> QPIFLNVLEAIEPGVVCAGHDNNQPDSFAALLSSLNELGERQLVHVVKWAKALPGFRNLHVDDQMAVIQYSWMGLMVFAMGWRSFTNVNSAMLYFAPDLVFNEYRMHKSRMYSQCVRMRHLSQEFGWLQITPQEFLCMKALLLFSIIPVDGLK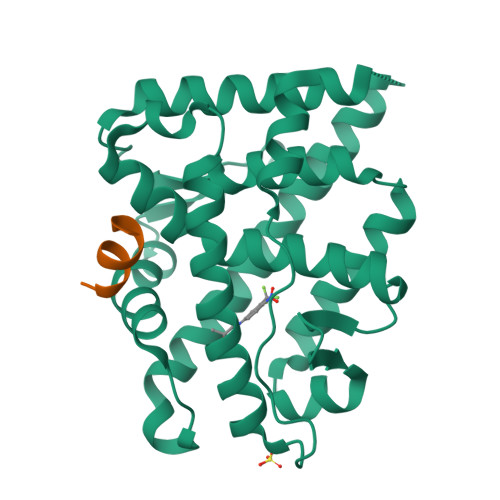NQKFFDELRMNYIKELDRIIACKRKNPTSCSRRFYQLTKLLDSVQPIARELHQFAFDLLIKSHMVSVDFPEMMAEIISVQVPKILSGKVKPIYFHTQ;> RGAFQNLFQSV> AISIKTPEDIEKMRVAGRLAAEVLEMIEPYVKPGVSTGELDRICNDYIVNEQHAVSACLGYHGYPKSVCISINEVVCHGIPDDAKLLKDGDIVNIDVTVIKDGFHGDTSKMFIVGKPTIMGERLCRITQESLYLALRMVKPGINLREIGAAIQKFVEAEGFSVVREYCGHGIGRGFHEEPQVLHYDSRETNVVLKPGMTFTIEPMVNAGKKEIRTMKDGWTVKTKDRSLSAQYEHTIVVTDNGCEILTLRKDDTIPAIISHDE

Methionine aminopeptidase (MetAP) removes the N-terminal methionine residue from nascent proteins in all types of cells. MetAP is therefore a potential target for developing novel broad spectrum antibacterial drugs. E. coli MetAP is a typical bacterial MetAP, containing only a catalytic domain. A surface-exposed loop containing Y62, H63, G64 and Y65 (the YHGY loop) is an integral part of the active site pocket.

We report here five new X-ray crystal structures of the Mn(II)-form of E. coli MetAP, each complexed with a different inhibitor. All eight structures, including the five new ones, have the typical "pita-bread" fold found in other MetAP structures, and each of them contains two Mn(II) ions at the dinuclear metal site. A single molecule of inhibitor sits in the shallow active site pocket. Common features of the Mn(II)-form selective inhibitors 4–8 bound to E. coli MetAP in the five new structures are that all use their carboxylate group to coordinate with the two Mn(II) ions at the dinuclear metal site and all take a non-coplanar or twisted conformation for the two aromatic rings, consistent with our previously reported structures of E. coli MetAP complexed with 1–3. The twisted conformation found in all of the Mn(II)-form-selective inhibitors 1–8 is in agreement with the requirement of a hydrophobic ortho-substitution, such as chlorine, on the phenyl ring for inhibitory activity. The twist angles observed in the MetAP complexes of 1–8 range from the smallest 23.3° for 6 to the largest 52.9° for 4, suggesting that in general, the phenylfuran-based inhibitors dock into the active site in a conformation that may correspond to a minimum-energy solution conformation. The residues forming the dinuclear metal site (H171, D108, E204, E235 and D97), as well as the nearby residues S110, T202, F177, H178 and H79, show little change in position upon binding of any of these inhibitors. In contrast, residues Y62, H63, G64, and Y65 in the YHGY loop, as well as residue W221, moved significantly. The same is true for other inhibitors, and the loop show a great adaptability. This flexibility allows the binding pocket to adapt to different shapes of the bound inhibitors.>MYYLGKELQKRSEELSRGFYELVYPPVDMYEEGGYLVVVADLAGFNKEKIKARVSGQNELIIEAEREITEPGVKYLTQRPKYVRKVIRLPYNVAKDAEISGKYENGVLTIRIPIAGT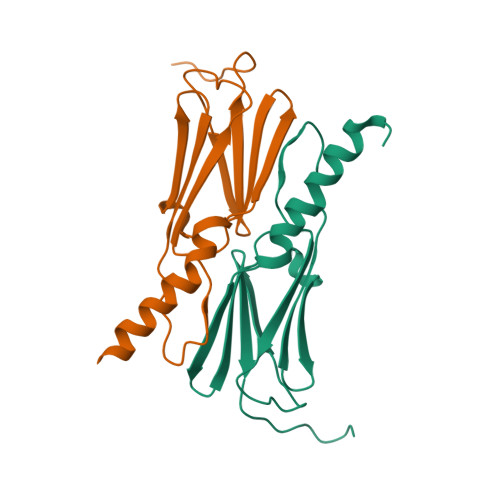SVFKFE[2x]> XCVIFPVEIDVSQTIIRDCQVDKQTRELVYINKIMNTQLTKPVLMM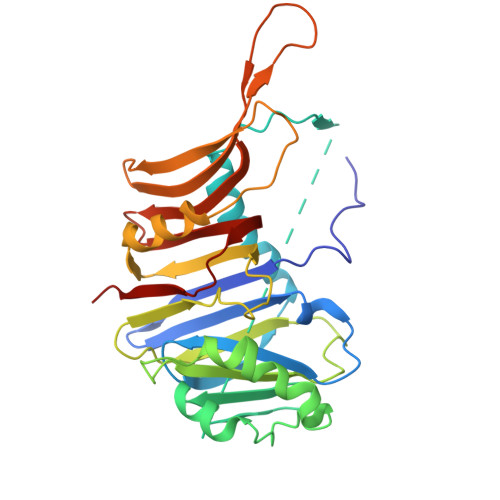FNISGPIRSVTRKNNNLRDRIKSKVDEQFDQLERDYSDQMDGFHDSIKYFKDEHYSVSCQNGSVLKSKFAKILKSHDYTDKKSIEAYEKYCLPKLVDERNDYYVAVCVLKPGFENGSNQVLSFEYNPIGNKVIVPFAHEINDTGLYEYDVVAYVDSVQFDGEQFEEFVQSLILPSSFKNSEKVLYYNEASKNKSMIYKALEFTTESSWGKSEKYNWKIFCNGFIYDKKSKVLYVKLHNVTSALNKNVILNTIK> MHHHHHHSSGRENLYFQGKERRRAVLELLQRPGNARCADCGAPDPDWASYTLGVFICLSCSGIHRNIPQVSKVKSVRLDAWEEAQVEFMASHGNDAARARFESKVPSFYYRPTPSDCQLLREQWIRAKYERQEFIYPEKQEPYSAGYREGFLWKRGRDNGQFLSRKFVLTEREGALKYFNRNDAKEPKAVMKIEHLNATFQPAKIGHPHGLQVTYLKDNSTRNIFIYHEDGKEIVDWFNALRAARFHYLQVAFPGASDADLVPKLSRNYLKEGYMEKTGPKQTEGFRKRWFTMDDRRLMYFKDPLDAFARGEVFIGSKESGYTVLH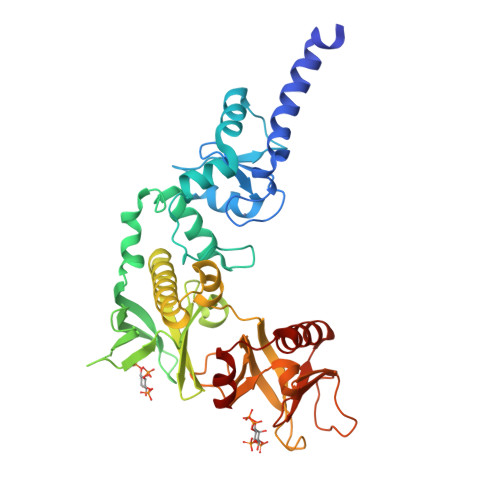GFPPSTQGHHWPHGITIVTPDRKFLFACETESDQREWVAAFQKAVDRPMLPQEYAVEAHF> GAMTFTRYSRLRVIAEIRHGDIFHSANIVSSIEFSDRDDELFATAGVSRCIKVFDFSSVVNEPADMQCPIVEMSTRSKLSCLSWNKHEKNHIASSDYEGIVTVWDVTTRQSLMEYEEHEKRAWSVDFSRTEPSMLVSGSDDCKVKVWCTRQEASVINIDMKANIC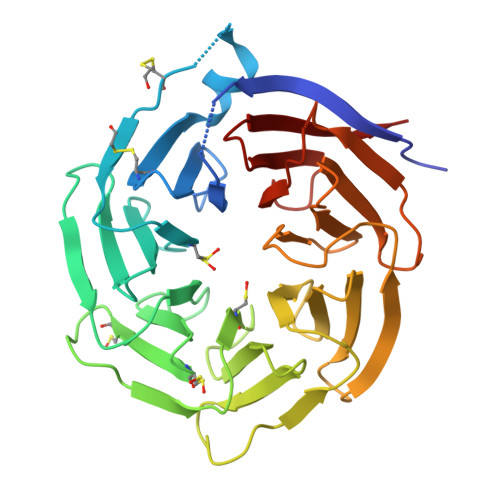CVKYNPGSSNYIAVGSADHHIHYYDLRNISQPLHVFSGHKKAVSYVKFLSNNELASASTDSTLRLWDVKDNLPVRTFRGHTNEKNFVGLTVNSEYLACGSETNEVYVYHKEITRPVTSHRFGSPDMDDAEEEAGSYFISAVCWKSDSPTMLTANSQGTIKVLVLAA>[2x]GPAMASKSPSEEVYPVKAFGLAAKDSSGLFSPFNFSRRATGEHDVQLKVLYCGTCQYDREMSKNKFGFTSYPYVLGHEIVGEVTEVGSKVQKFKVGDKVGVASIIETCGKCEMCTNE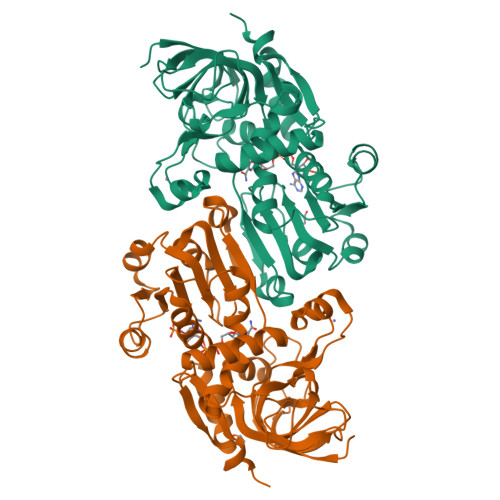VENYCPEAGSIDSNYGACSNIAVINENFVIRWPENLPLDSGVPLLCAGITAYSPMKRYGLDKPGKRIGIAGLGGLGHVALRFAKAFGAKVTVISSSLKKKREAFEKFGADSFLVSSNPEEMQGAAGTLDGIIDTIPGNHSLEPLLALLKPLGKLIILGAPEMPFEVPAPSLLMGGKVMAASTAGSMKEIQEMIEFAAEHNIVADVEVISIDYVNTAMERLDNSDVRYRFVIDIGNTLKSN> AVSLDRTRAVFDGSEKSMTLDISNDNKQLPYLA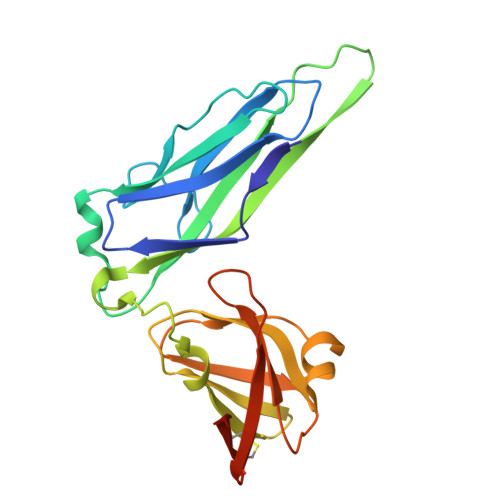QAWIENENQEKIITGPVIATPPVQRLEPGAKSMVRLSTTPDISKLPQDRESLFYFNLREIPPRSEKANVLQIALQTKIKLFYRPAAIKTRPNEVWQDQLILNKVSGGYRIENPTPYYVTVIGLGGSEKQAEEGEFETVMLSPRSEQTVKSANYNTPYLSYINDYGGRPVLSFICNGSRCSVKKEKHHHHHH>MRGSHHHHHHGSMASKVESRQAAVLAIATANPPNIFYQADYPDFYFRVTKSEHMTQLKDKFKRMCEKSMIRKRHMYLTEDVIKENPNIGILNAPSFNARQEIMVEEVPKLGKEAALKAIKEWGQPLSKLTHLIFCTSSGVNMPSADYHLAKIMGLPPYVQRTMIYQQGCFAGATALRLAKDIAENNGGHTRILIVCVELMVVCFQAPSDTYLDLLVGNAIFSDGAAAAIVGADLDTTTERPIFNIVSANQTTIPDSEDGIVGHIREMGMKYYLSRTVPQVIGNNIVQCCRDTFTPLGINDWNSMFYIVHPGGPAVLRMMEEKLGLSKERMRASWHVLSEYG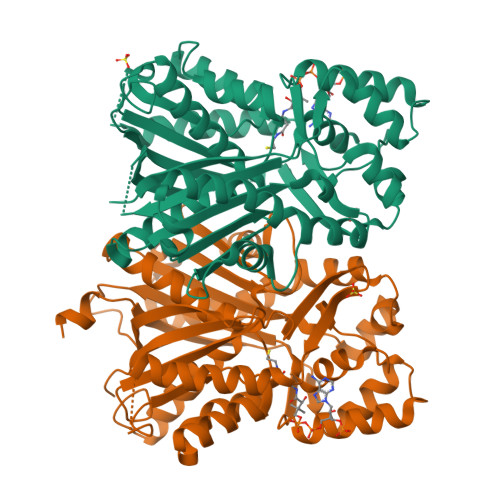NMQGPSVLFILDEMRNKSMEEGKSTTGEGLEWGVMFGFGPGLTVETVVLRSVAIN[4x]N-{3-[(4S,6S)-2-amino-4-(fluoromethyl)-6-(trifluoromethyl)-5,6-dihydro-4H-1,3-oxazin-4-yl]-4-fluorophenyl}-5-cyanopyridine-2-carboxamide | C19 H14 F5 N5 O2 | 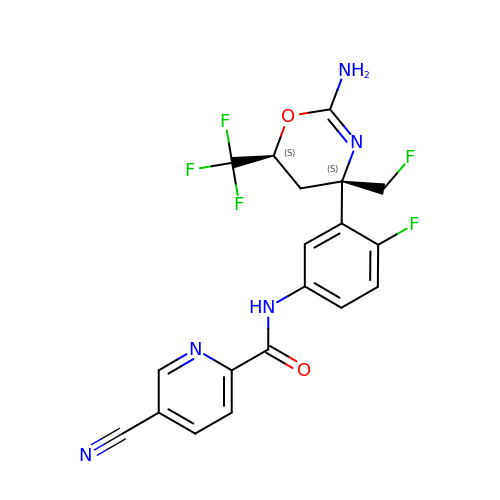QCMXWFUAVCHHIA-MAUKXSAKSA-N> MYKDLKFPVLIVHRDIKADTVAGERVRGIAHELEQDGFSILSTASSAEGRIVASTHHGLACILVAAEGAGENQRLLQDVVELIRVARVRAPQLPIFALGEQVTIENAPAESMADLHQLRGILYLFEDTVPFLARQVARAARNYLAGLLPPFFRALVEHTAQSNYSWHTPGHGGGVAYRKSPVGQAFHQFFGENTLRSDLSVSVPELGSLLDHTGPLAEAEDRAARNFGADHTFFVINGTSTANKIVWHSMVGREDLVLVDRNCHKSILHSIIMTGAIPLYLTPERNELGIIGPIPLSEFSKESIAAKIAASPLARGREPKVKLAVVTNSTYDGLCYNAELIKQTLGDSVEVLHFDEAWYAYAAFHEFYDGRYGMGTSRSEEGPLVFATHSTHKMLAAFSQASMIHVQDGGTRKLDVARFNEAFMMHISTSPQYGIIASLDVASAMMEGPAGRSLIQETFDEALSFRRALANVRQNLDRNDWWFGVWQPEQVEGTDQVGTHDWVLEPSADWHGFGDIAEDYVLLDPIKVTLTTPGLSAGGKLS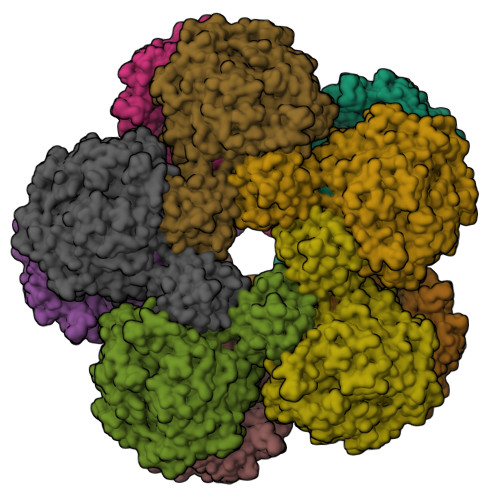EQGIPAAIVSRFLWERGLVVEKTGLYSFLVLFSMGITKGKWSTLVTELLEFKRCYDANLPLLDVLPSVAQAGGKRYNGVGLRDLSDAMHASYRDNATAKAMKRMYTVLPEVAMRPSEAYDKLVRGEVEAVPIARLEGRIAAVMLVPYPPGIPLIMPGERFTEATRSILDYLEFARTFERAFPGFDSDVHGLQHQDGPSGRCYTVECIKE> UGCCUGGCGGC;> CCG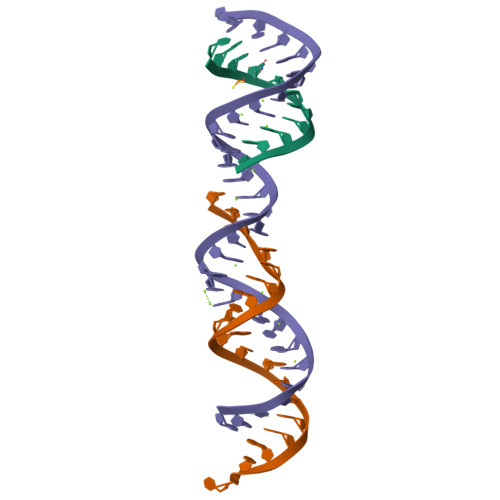AUGGUAGUGUGGGGUC;> CCCCAUGCGAGAGUAGGGAACUGCCAGGCAU> KNHSINHDLDTSFINFAPKNLKLLDPKQFPQGEILKALPLLKNESKEKNIFHATLEIKENHIELIKGKKTLFYTYNGLVPAPKIEVFEGDKLEILVKNKLKEATTIHWHGVPVPPDQDGSPHDPILAGEERIYRFEIPQDSAGTYWYHPHPHYTASKQVFMGLAGAFVIKAKKDALSHLKEKDLMISDLRLDENAQIPNNNLNDWLNGREGEFVLINGQFKPKIKLATNERIRIYNATAARYLNLRIQGAKFILVGTDGGLIEKTIYKEELFLSPASRVEVLIDAPKDGNFKLESAYYDRDKMMVKEEPNTLFLANINLKKENVELPKNLKIFKPSEEPKEFKEIIMSEDHMQMHGMMGKSEGELKIALASMFLINRKSYDLKRIDLSSKLGVVEDWIVINKSHMDHPFHIHGTQFELISSKLNGKVQKAEFRALRDTINVRPNEELRLRMKQDFKGLRMYHCHILEHEDLGMMG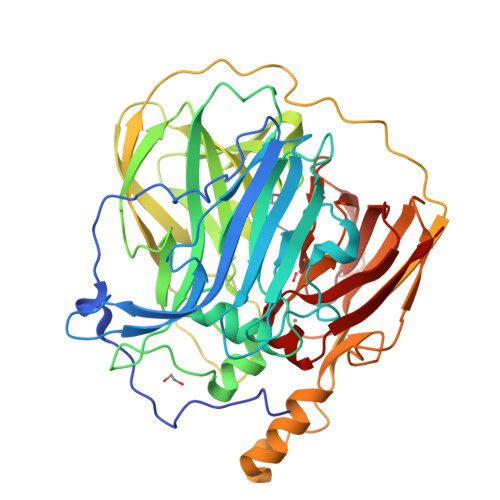NLEVKE(R)-4-((R)-3-amino-4-(2,4,5-trifluorophenyl)butanoyl)-3-(tert-butoxymethyl)piperazine-2-one | C19 H26 F3 N3 O3 | 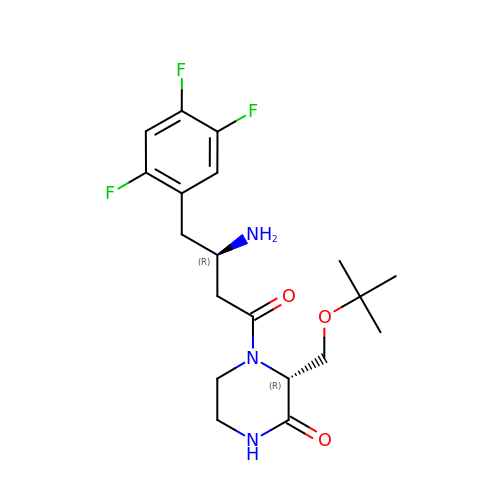LCDDAGSJHKEABN-MLGOLLRUSA-N> GMGFSSELCSPQGHGVLQQMQEAELRLLEGMRKWMAQRVKSDREYAGLLHHMSLQDSGGQSRAISPDSPISQSWAEITSQTEGLSRLLRQHAEDLNSGPLSKLSLLIRERQQLRKTYSEQWQQLQQELTKTHSQDIEKLKSQYRALARDSAQAKRKYQEASKDKDRDKA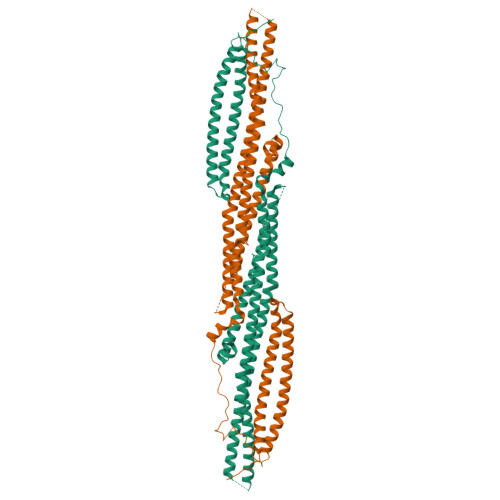KDKYVRSLWKLFAHHNRYVLGVRAAQLHHQHHHQLLLPGLLRSLQDLHEEMACILKEILQEYLEISSLVQDEVVAIHREMAAAAARIQPEAEYQGFLRQYGSAPDVPPCVTFDESLLEEGEPLEPGELQLNELTVESVQHTLTSVTDELAVATEMVFRRQEMVTQLQQELRNEEENTHPRERVQLLGKRQVLQEALQGLQVALCSQAKLQAQQELLQTKLEHLGPGEPPPVLLLQDD> MAQILPIRFQEHLQLQNLGINPANIGFSTLTMESDKFICIREKVGEQAQVVIIDMNDPSNPIRRPISADSAIMNPA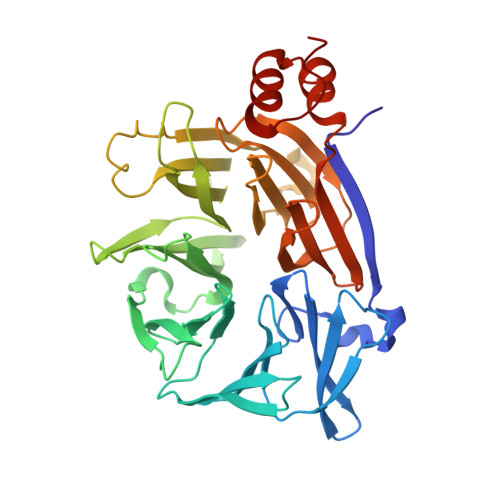SKVIALKAGKTLQIFNIEMKSKMKAHTMTDDVTFWKWISLNTVALVTDNAVYHWSMEGESQPVKMFDRHSSLAGCQIINYRTDAKQKWLLLTGISAQQNRVVGAMQLYSVDRKVSQPIEGHAASFAQFKMEGNAEESTLFCFAVRGQAGGKLHIIEVGTPPTGNQPFPKKAVDVFFPPEAQNDFPVAMQISEKHDVVFLITKYGYIHLYDLETGTCIYMNRISGETIFVTAPHEATAGIIGVNRKGQVLSVCVEEENIIPYITNVLQNPDLALRMAVRNNLAGAEELF> SNAMPFLRPRYVLVLIALFGTVCGSLSGCVQKKS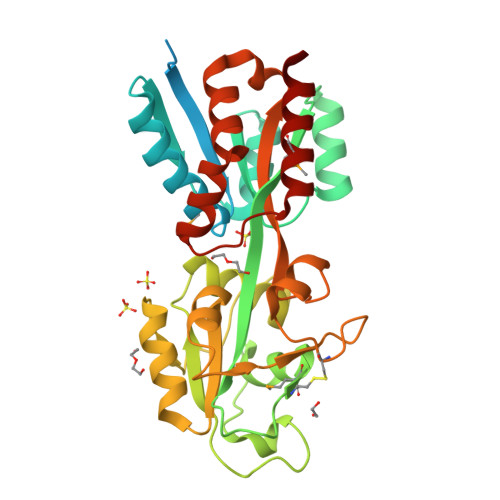ADQAASTSEKTNSSTEGMNAATPSISGTIAVDGSSTVFPISQAVAEEFEGKFPEVKLTVAMSGTGGGFKKFIAEEIDVTGASRPITEKEAAECKAKGIDYVEFQVAIDGLTVVINPANTFAECMTVAELNKIWAADSKVSKWSEVREGWPDEPIQLFGADTASGTFDYFTEVINGKAKSSRSDYTANSNDNILVQGVVDSKGALGYFGYAYFAENASKLKAVKISDGKKAVCVEPTPATIESGEYTPLSRPLFIYTTKAKLKRPEVAEFIKFLLSEKGDQLVEEVKYIKVPKSVKETMQQRLADALK>[2x]MDEGMWLMQQLGRKYAQMKERGLKMKEYDLYNPNGTSLKDAVVLFDGGCTGEVVSDRGLVLTNHHCGYDMIQAHSTL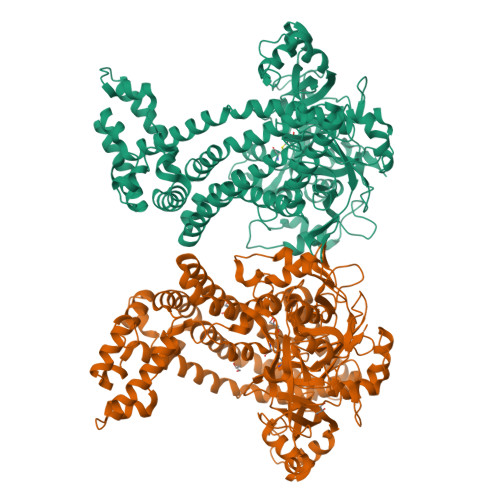EHNYLENGFWAMREADELPNKDISVVFIDKIEDVTDYVKKELKAIKDPNSMDYLSPKYLQKLADKKAGKNFSAKNPGLSVEIKAFYGGNLYLMFTKKTYTDVRLVGAPPSSIGKFGADTDNWIWPRHTGDFSIFRIYADKNGNPAPYSEDNVPLKPKRFFNISLGGVQENDYAMIMGFPGTTHRYFTASEVDEWKSIDNDIRIRMRDIRQGVMLREMLADPQIKIMYSAKYAASQNAYKRAIGANWAIKTRGLRQNKQAMQDRLIAWGAKQGTPRYEEAVHEIDATVAKRADLRRRYWMIEEGIIRGIEFARSPIPTEDETKALQGNDASARKEAIDKIRTRYSKFANKDYSAEVDKKVAVAMLTEYLKEIPYENLPLHLRLVKDRFAGDVQAYVDDIFARSVFGSEAQFDAFAAVPSVEKLAEDPMVLFASSVFDEYRKLYNELRPYDDPILRAQRTYIAGLLEMDGDQDQFPDANLTLRFTYGQVKGYSPRDNVYYGHQTTLDGVMEKEDPDNWEFVVDPKLKAVYERKDFGRYADRSGRMPVAFCATTHTTGGNAGSPVMNANGELIGLNFDRNWEGVGGDIQYLADYQRSIIVDIRYVLLVIDKVGGCQRLLDEMNIVPHHHHHH> GPMATVFRQENVDDYYDTGEELGSGQFAVVKK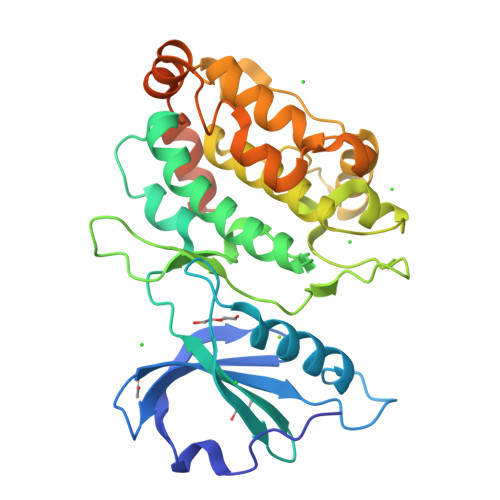CREKSTGLQYAAKFIKKRRTKSSRRGVSREDIEREVSILKEIQHPNVITLHEVYENKTDVILILELVAGGELFDFLAEKESLTEEEATEFLKQILNGVYYLHSLQIAHFDLKPENIMLLDRNVPKPRIKIIDFGLAHKIDFGNEFKNIFGTPEFVAPEIVNYEPLGLEADMWSIGVITYILLSGASPFLGDTKQETLANVSAVNYEFEDEYFSNTSALAKDFIRRLLVKDPKKRMTIQDSLQHPWIKPKDTQQALSRKAAAVNMEKFKKFAARKKWKQEVRLISLCQRLSRSFLSRSNMSVARSD Here, we identify an evolutionarily conserved hexapeptide sequence as the major aggregation-prone region (APR) of gastrointestinal peptides of the glucagon family: xFxxWL. We determine nine polymorphic crystal structures of the APR segments of glucagon-like peptides 1 and 2, and exendin and its derivatives. We propose that the pH-dependent changes of the protonation states of glutamate/aspartate residues of APRs initiate switching between the amyloid and the folded, monomeric forms of the hormones. Our results highlight the dual role of short aggregation core motifs in reversible amyloid formation and receptor binding.

Crystals of APRGLP1 grew only at a low pH (pH ≈ 2, T = 37 °C) where the N-terminal glutamic acid self-converted to a pyroglutamic acid (pE) via a spontaneous ring closure. In the structure of APRGLP1 the hydrophobic residues (Phe, Ile, Ala, Leu) form a hydrophobic core, while Trp and pGlu participate in H-bonding with each other and water molecules. In the crystal structure of pEFIAWL, the ring-closure of an N-terminal Glu residue (resulting in the formation of pyroglutamic acid) makes the N-terminal more hydrophobic by eliminating the charge frustrations linked to both the Glu side chain and the protonated N-terminal amine. The crystal structure of APRGLP1 provide an example where pyroglutamic acid built in a β-spine amyloid nanostructure can be studied. Based on our current results, we propose that the elimination of the charges by ring closure, significantly contributes to self-assembly, compared to sole side chain protonation of Glu. This might also be the reason why we observed the presence of pEFIAWL in the crystal state while the parent hexapeptide, EFIAWL, did not crystallize despite forming amyloid. The five-membered ring structure of pGlu shows similar geometry to that of Pro, which is considered a formidable β-sheet breaker. Thus, cyclic pGlu with quasi-fixed dihedrals would be expected to function as a gatekeeper of amyloid formation by twisting the backbone structures away from that of typical β-strands. However, the example of the crystal structure of pEFIAWL provides compelling evidence that a Pro-like residue right next to an APR does not necessarily prevent β-stranded amyloid formation. The glucagon-like APRs (APRGLP2 and APRGLP1) show an extensive contact surface (Sc = ~0.80; Area = ~160 Å2) along the extended, linear backbone of high complementarity, while exendin-like sequences (APRex-4 and APRTc5b) present generally smaller values (Sc = ~0.65; Area = ~110 Å2).

> QFIAWL>[4x]MKTIGLLGGMSWESTIPYY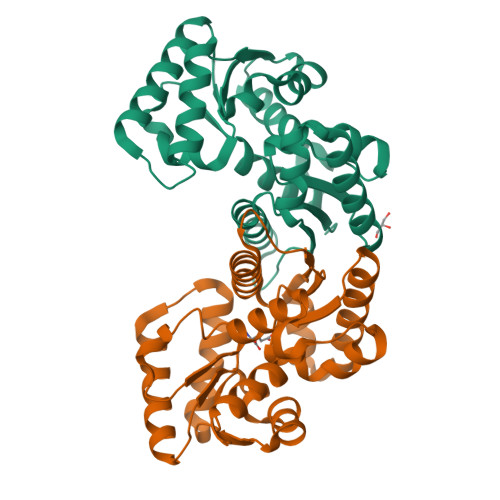RLINEGIKQRLGGLHSAQVLLHSVDFHEIEECQRRGEWDKTGDILAEAALGLQRAGAEGIVLCTNTMHKVADAIESRCTLPFLHIADATGRAITGAGMTRVALLGTRYTMEQDFYRGRLTEQFSINCLIPEADERAKINQIIFEELCLGQFTEASRAYYAQVIARLAEQGAQGVIFGSTEIGLLVPEERSVLPVFDTAAIHAEDAVAFMLSLEHHHHHH>[2x]GAMAMNGEAICSALPTIPYHKLADLRYLSRGAS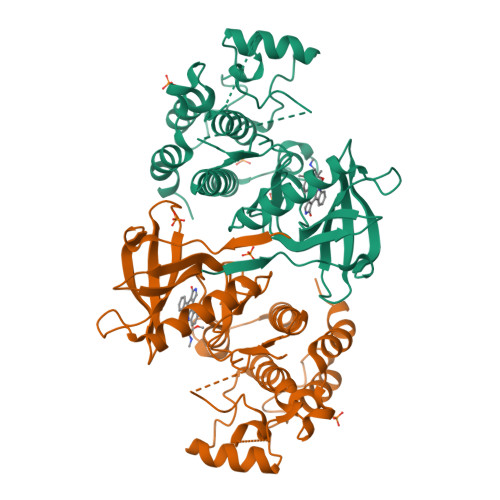GTVSSARHADWRVQVAVKHLHIHTPLLDSERKDVLREAEILHKARFSYILPILGICNEPEFLGIVTEYMPNGSLNELLHRKTEYPDVAWPLRFRILHEIALGVNYLHNMTPPLLHHNLKTQNILLDNEFHVKIADFGLSKWRMMSLSQSRSSKSAPEGGTIIYMPPENYEPGQKSRASIKHDIYSYAVITWEVLSRKQPFEDVTNPLQIMYSVSQGHRPVINEESLPYDIPHRARMISLIESGWAQNPDERPSFLKCLIELEPVLRTFEEI Gloeobacter violaceus proton-gated ion channel (GLIC), a prokaryotic model of pLGICs, is particularly well-suited to stabilize preactive states under suboptimal activating conditions modulated by pH. The GLIC homomer consists of five subunits, each with an ECD and TMD. GLIC is activated by the protonation of a series of titratable residues in the ECD, leading to counterclockwise rotation and contraction of the ECD. Therefore, we established a data processing strategy involving symmetry expansion, backtracking particles, supervised particle reorientation, and 3D reconstruction to resolve high-resolution maps of various asymmetric intermediate states of nanodisc-reconstituted GLIC at pH 4.0, which provide comprehensive understanding of activation mechanism of GLIC.

To explore this, we prepared a nanodisc-embedded GLIC-Y251A mutant at pH 2.5 for cryo-EM analysis. Although only a homopentameric configuration was previously resolved at this pH for the WT, focused classification of GLIC-Y251A mutant unexpectedly revealed that 44% of the subunits adopt the o conformation, while the remaining subunits adopt the i conformation. Interestingly, only 2.2% of the population adopt the o5 state whereas 11.3% of the population adopt i1o4 state. Particles corresponding to i1o4 state were reconstructed to a map with nominal resolution of 2.87 Å, with clear densities across all regions. Comparison of the atomic model of GLIC-Y251A i1o4 built into the cryo-EM map with GLIC-WT i1o4 shows similar conformation with backbone RMSDCα of 0.40 Å and similar pore profile. Therefore, the functional profile of GLIC-Y251A i1o4 should resemble the GLIC-WT i1o4 which is partially conductive. The pronounced reduction of the o5 state in Y251A, even at pH 2.5, compared to WT at pH 4.0, indicates a drastic shift in activation equilibrium. This suggests that Y251 is essential for stabilizing the outward conformation of the M2–M3 loop in coordination with the outward displacement of F116. Our cryo-EM data yielded unexpected results with 86.5% nonconductive channels, 11.3% partially conductive channels and only 2.2% conductive channels, which suggests that the Y251A mutation reduces the channel conductivity significantly. These findings suggest that Y251 plays a crucial role in gating by stabilizing the outward M2–M3 loop conformation (o).

>[5x]VSPPPPIADEPLTVNTGIYLIECYSLDDKAETFKVNAFLSLSWKDRRLAFDPVRSGVRVKTYEPEAIWIPEIRFVNVENARDADVVDISVSPDGTVQYLERFSARVLSPLDFRRYPFDSQTLHIYLIVRSVDTRNIVLAVDLEKVGKNDDVFLTGWDIESFTAVVKPANFALEDRLESKLDYQLRISRQYFSYIPNIILPMLFILFISWTAFWSTSYEANVTLVVSTLIAHIAFNILVETNLPKTPAMTYTGAIIFMIYLFYFVAVIEVTVQHYLKVESQPARAASITRASRIAFPVVFLLANIILAFLFFG5-(3-fluorophenyl)-N-[(3S)-3-piperidyl]-3-ureido-thiophene-2-carboxamide 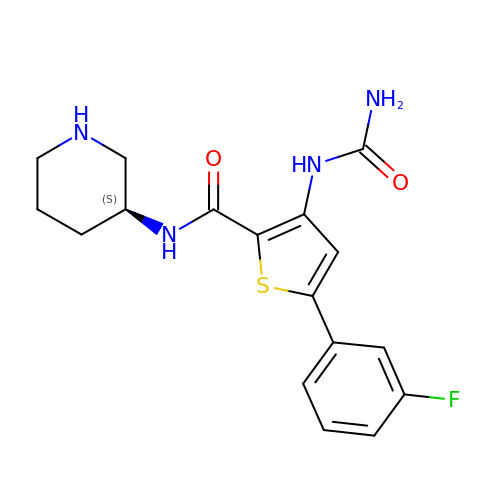| C17 H19 F N4 O2 S | IAYGCINLNONXHY-LBPRGKRZSA-N>HHHHHHFNLPPGNYKKPVLLYSSSGGHFLRILPDGTVDGTRDRSDQHIQLQLSAESVGEVYIKSTETGQYLAMDTDGLLYGSQTPNEECLFLERLEENHYNTYISKKHAEKNWFVGLKKNGS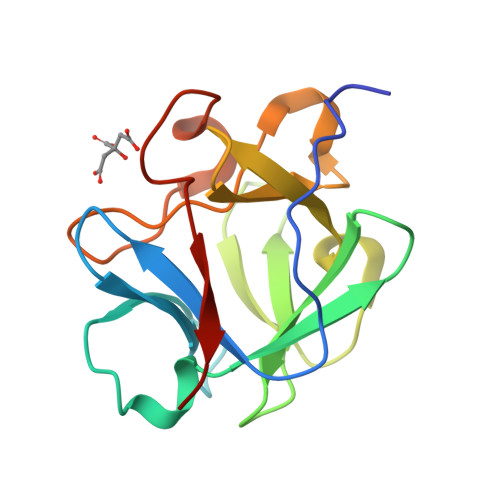VKRGPRTHYGQKAILFLVLPVSSD[2x]>[2x]AQLTTESMPFNVAEGKEVLLLVHNLPQQLFGYSWYKGERVDGNR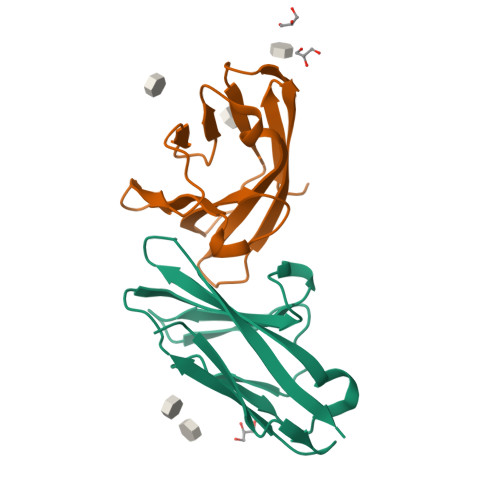QIVGYAIGTQQATPGPANSGRETIYPNASLLIQNVTQNDTGFYTLQVIKSDLVNEEATGQFHVY>MATAQVTCVWDLKATLGEGPIWHGDTLWFVDIKQRKIHNYHPATGERFSFDAPDQVTFLAPIVGATGFVVGLKTGIHRFHPATGFSLLLEVEDAALNNRPNDATVDAQGRLWFGTMHDGEENNSGSLYRMDLTGVARMDRDICITNGPCVSPDGKTFYHTDTLEKTIYAFDLAEDGL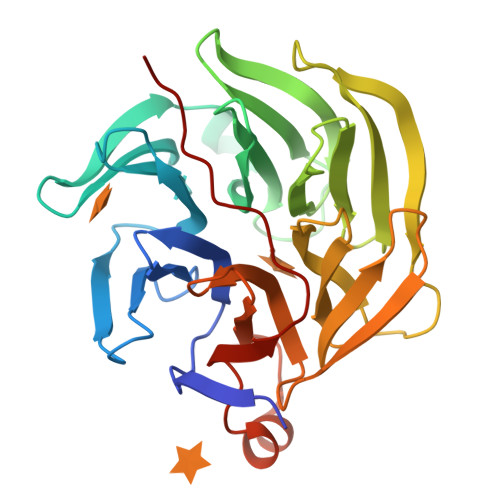LSNKRVFVQFALGDDVYPDGSVVDSEGYLWTALWGGFGAVRFSPQGDAVTRIELPAPNVTKPCFGGPDLKTLYFTTARKGLSDETLAQYPLAGGVFAVPVDVAGQPQHEVRLV[4x]>[2x]MGQRGQVCQGKCMAEDQQSSQISDTVPALRRAVRILDLVAGSPRDLTAAELTRFLDLPKSSAHGLLAVMTELDLLARSADGTLRIGPHSLRWANGFLSHLDIVSTFNDHLAQRHDLDPYTVTLTVREGGEVVYIGCRNSAQPLGHTFRIGMRLPAPFTATGKILLSDLGPGELRMLFSQFPQPLTSRSVAGLSQLEE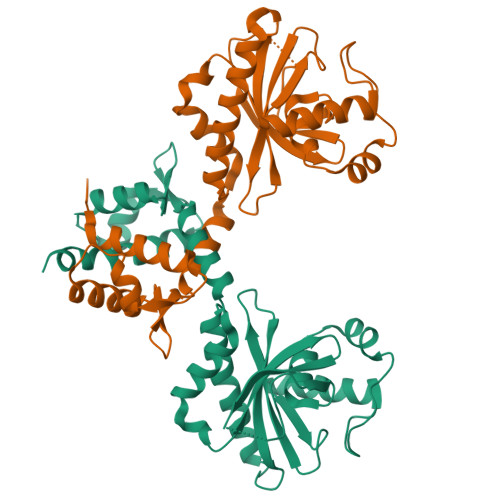ELALTRARGYSIDDGQIREGMLCIGAAIRDYSGAASAGIAISLIRSEASDEKIAYLGEELRTTANALSEKLGYRSQKD> TEVLWPAVPNGTDAAFLAGPGSSWGNSTVASTAAVSSSFKCALTKTGFQFYYLPAVYILVFIIGFLGNSVAIWMFVFHMKPWSGISVYMFNLALADFLYVLTLPALIFYYFNKTDWIFGDAMCKLQRFI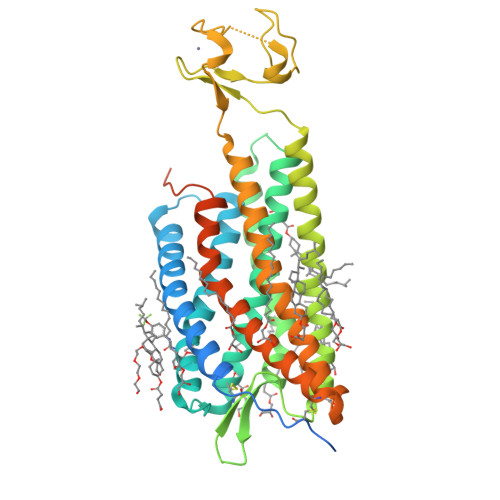FHVNLYGSILFLTCISAHRYSGVVYPLKSLGRLKKKNAICISVLVWLIVVVAISPILFYSGTGVRKNKTITCYDTTSDEYLRSYFIYSMCTTVAMFCVPLVLILGCYGLIVRALIYKMKKYTCTVCGYIYNPEDGDPDNGVNPGTDFKDIPDDWVCPLCGVGKDQFEEVEEPLRRKSIYLVIIVLTVFAVSYIPFHVMKTMNLRARLDFQTPAMCAFNDRVYATYQVTRGLASLNSCVNPILYFLAGDTFRRRLSRATRKASRRSEANLQSKSEDMTLNILPEFKQNGDTSL>MDKKELFDTVINLEEQIGSLYRQLGDLKQHIGEMIEENHHLQLENKHL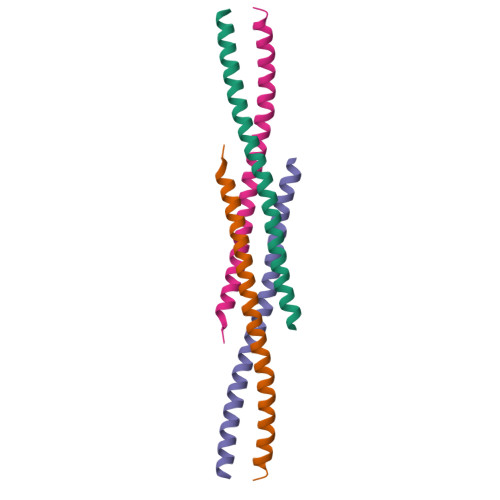RKRLDDTTQQIEKF[2x]>[2x]MTTTLLAVNGTLMRGLELNPNMQKAGGIFVREDRTDAHYRLWSINDRHPGMIRVNEGGTHVDVEIWQLPLASF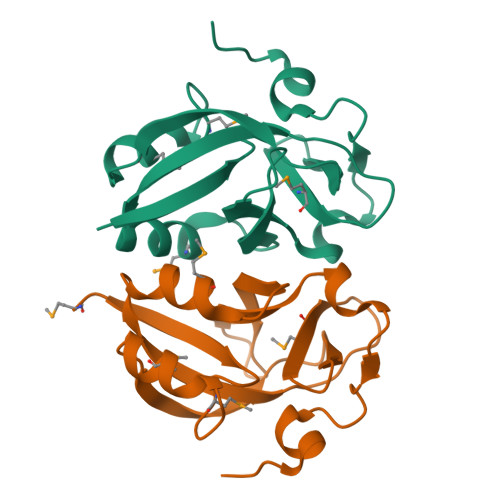AALLMSEPAGLAIGKIKLADGSEVLGVLAENWLTEGQREITELGSWRKYTGHFHTVLEHHHHHH>[6x]MLRTMLKSKIHRATVTCADLHYVG;>[6x]XVTIDA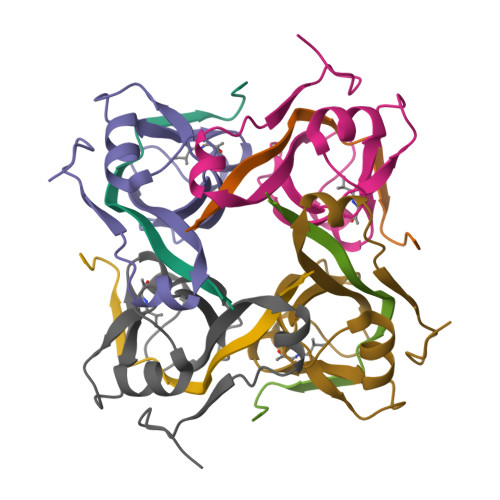DLMDAADLLEGEQVTIVDIDNGARLVTYAITGERGSGVIGINGAAAHLVHPGDLVILIAYATMDDARARTYQPRIVFVDAYNKPIDMGHDPAFVPENAGELLDPRLGVGLEHHHHHH> MKLNIAYPRNGTVKQFEISDEVLRRVQLQDYRLGNEVDGAIFGSEFKGYIFRLRGGSDKDGFPMVPGVLASSRVSLLVKRGAIGFNTFRGYQGERRRKNVRGCVLASDIALVNVTISKVGDQPIEGVTDTTAPRRLGPKRASKIRK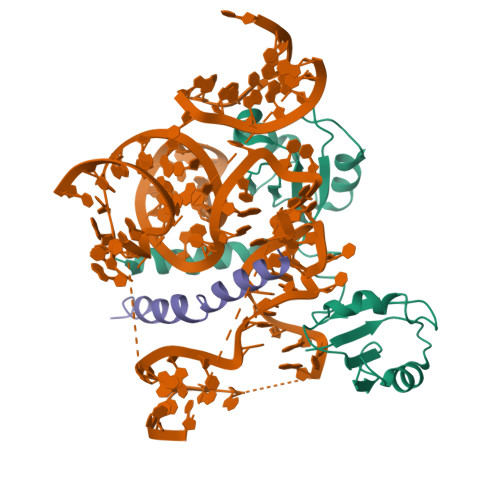LFNLSRTEDVRKYVVRRRVVKSGKKDRLKAPKIQRLITPRVKARRAKKAKDAIAKVRASAAERREYLRLIASNRRALRQRDHSKKHTRKVHAQRAEVAAFQKK;> MPAKAAAKPVKPATKAAPKPANKAPAPKAAAAKPVAKAAPKAAAPAVRPASGSSNGVYVKNWGTGSVADATNVFSAAGKVVKVQLRRQRYALVFFENSAAVKKAIDLFNEKEVLGQTVLVVPAKASPKPDAHENSSCVFVSPIFRPSTTKAQVMELFAGVKVQRLRMYRQNFAYAYLDSPAAAKKFVEEKNGTAFRGHTLRVALSARSLEKLRARQEVANVVIAAHRHYKVHERQ>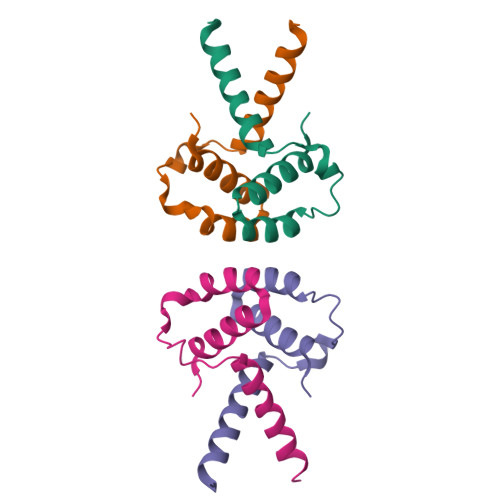MSITSDEVNFLVYRYLQESGFSHSAFTFGIESHISQSNINGTLVPPAALISILQKGLQYVEAEISINEDGTVFDGRPIESLSLIDAVMPD[12x]4-amino-8-(5-methyl-1H-indazol-6-yl)cinnoline-3-carboxamide | C17 H14 N6 O | 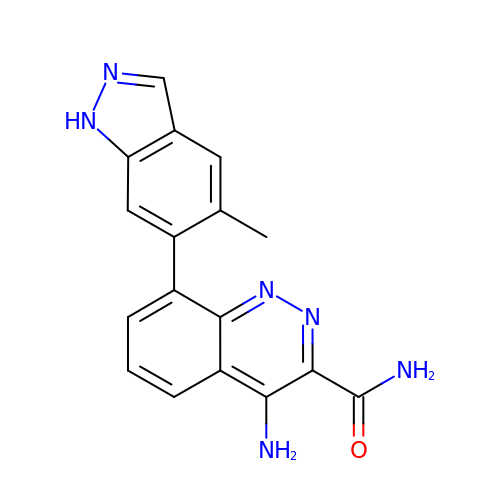PTHVKCSYXICMAR-UHFFFAOYSA-N> MSHQKIIQDLIAWIDEHIDQPLNIDVVAKKSGYSKWYLQRMFRTVTHQTLGDYIRQRRLLLAAVELRTTERPIFDIAMDLGYVSQQTFSRVFRR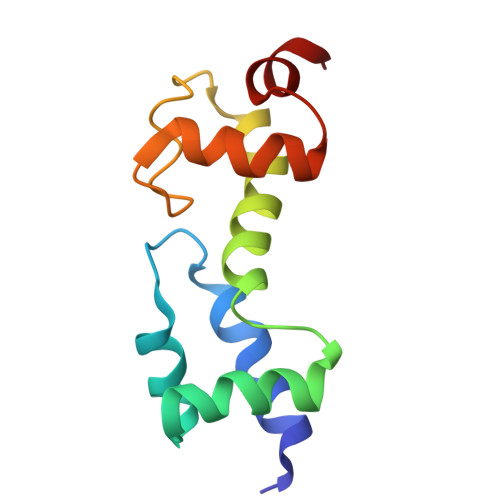QFDRTPSDYRHRL> MVQRWLYSTNAKDIAVLYFMLAIFSGMAGTAMSLIIRLELAAPGSQYLHGNSQLFNVLVVGHAVLMIFFLVMPALIGGFGNYLLPLMIGATDTAFPRINNIAFWVLPMGLVCLVTSTLVESGAGTGWTVYPPLSSIQAHSGPSVDLAIFALHLTSISSLLGAINFIVTTLNMRTNGMTMHKLPLFVWSIFITAFLLLLSLPVLSAGITMLLLDRNFNTSFFEVSGGGDPILYEHLFWFFGHPEVYILIIPGFGIISHVVSTYSKKPVFGEISMVYAMASIGLLGFLVWSHHMYIVGLDADTRAYFTSATMIIAIPTGIKIFSWLATIHGGSIRLATPMLYAIAFLFLFTMGGLTGVALANASLDVAFHDTYYVVGHFHYVLSMGAIFSLFAGYYYWSPQILGLNYNEKLAQIQFWLIFIGANVIFFPMHFLGINGMPRRIPDYPDAFAGWNYVASIGSFIATLSLFLFIYILYDQLVNGLNNKVNNKSVIYNKAPDFVESNTIFNLNTVKSSSIEFLLTSPPAVHSFNTPAVQS;> DVPTPYACYFQDSATPNQEGILELHDNIMFYLLVILGLVSWMLYTIVMTYSKNPIAYKYIKHGQTIEVIWTIFPAVILLIIAFPSFILLYLCDEVISPAMTIKAIGYQWYWKYEYSDFINDSGETVEFESYVIPDELLEEGQLRLLDTDTSMVVPVDTHIRFVVTAADVIHDFAIPSLGIKVDATPGRLNQVSALIQREGVFYGACSELCGTGHANMPIKIEAVSLPKFLEWLNEQ;> MTHLERSRHQQHPFHMVMPSPWPIVVSFALLSLALSTALTMHGYIGNMNMVYLALFVLLTSSILWFRDIVAEATYLGDHTMAVRKGINLGFLMFVLSEVLIFAGLFWAYFHSAMSPDVTLGACWPPVGIEAVQPTELPLLNTIILLSSGATVTYSHHALIAGNRNKALSGLLITFWLIVIFVTCQYIEYTNAAFTISDGVYGSVFYAGTGLHFLHMVMLAAMLGVNYWRMRNYHLTAGHHVGYETTIIYTHVLDVIWLFLYVVFYWWGV;> QQKPVVKTAQNLAEVNGPETLIGPGAKEGTVPTDLDQETGLARLELLGKLEGIDVFDTKPLDSSRKGTMKDPIIIESYDDYRYVGCTGSPAGSHTIMWLKPTVNEVARCWECGSVYKLNPVGVPNDDHHH;> AQTHALSNAAVMDLQSRWENMPSTEQQDIVSKLSERQKLPWAQLTEPEKQAVWYISYGEWGPRRPVLNKGDSSFIAKGVAAGLLFSVGLFAVVRMAGGQDAKTMNKEWQLKSDEYLKSKNANPWGGYSQVQSK;> SDAHDEETFEEFTARYEKEFDEAYDLFEVQRVLNNCFSYDLVPAPAVIEKALRAARRVNDLPTAIRVFEALKYKVENEDQYKAYLDELKDVRQELGVPLKEELFPSSS;> ANKVIQLQKIFQSSTKPLWWRHPRSALYLYPFYAI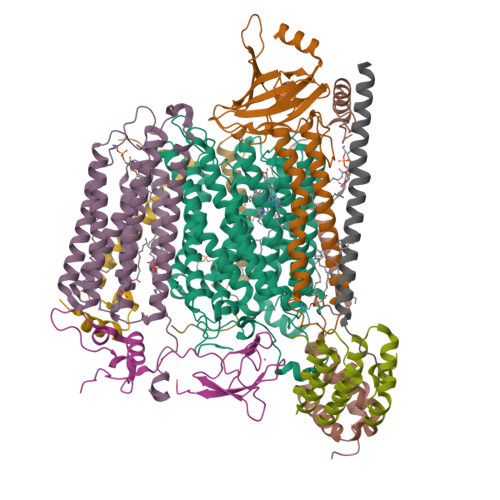FAVAVVTPLLYIPNAIRGIKAKKA;> VHFKDGVYENIPFKVKGRKTPYALSHFGFFAIGFAVPFVACYVQLKKSGAF;> TIAPITGTIKRRVIMDIVLGFSLGGVMASYWWWGFHMDKINKREKFYAELAERKK> CGGPFELWEPNTTFSSTNFPNSYPNLAFCVWILNAQKGKNIQLHFQEFDLENINDVVEIRDGEEADSLLLAVYTGPGPVKDVFSTTNRMTVLLITNDVLARGGFKANFTTGYHLGIPEPCKADHFQCKNGECVPLVNLCDGHLHCEDGSDEADCVRFFNGTTNNNGLVRFRI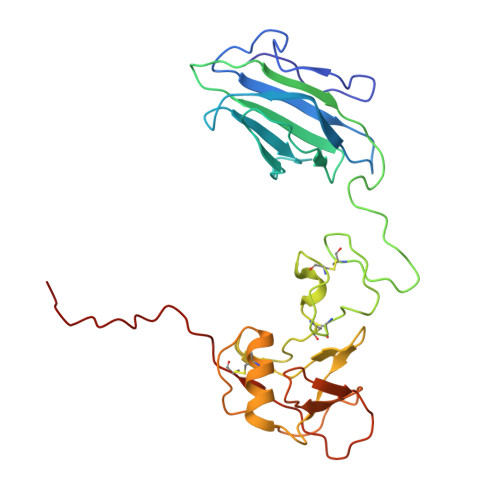QSIWHTACAENWTTQISNDVCQLLGLGSGNSSKPIFPTDGGPFVKLNTAPDGHLILTPSQQCLQDSLIRLQCNHKSCGKKLAAQDITPK>[28x]LMSDWEDEDLDTDNDNIPDSYERNGYTIKDLIAVKWEDSFAEQGYKKYVSNYLESNTAGDPYTDYEKASGSFDKAIKTEARDPLVAAYPIVGVGMEKLIISTNEHASTDQGKTVSRATTNSKTESNTAGVSVNVGYQNGFTANVTTNYSHTTDNSTAVQDSNGESWNTGLSINKGESAYINANVRYYNTGTAPMYKVTPTTNLVLDGDTLSTIKAQENQIGNNLSPGDTYPKKGLSPLALNTMDQFSSRLIPINYDQLKKLDAGKQIKLETTQVSGNFGTKNSSGQIVTEGNSWSDYISQIDSISASIILDTENESYERRVTAKNLQDPEDKTPELTIGEAIEKAFGATKK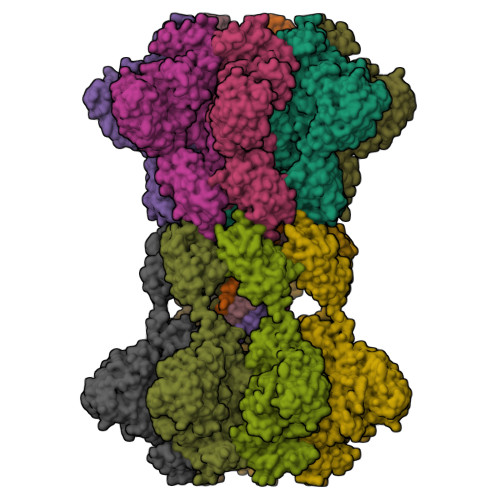DGLLYFNDIPIDESCVELIFDDNTANKIKDSLKTLSDKKIYNVKLERGMNILIKTPTYFTNFDDYNNYPSTWSNVNTTNQDGLQGSANKLNGETKIKIPMSELKPYKRYVFSGYSKDPLTSNSIIVKIKAKEEKTDYLVPEQGYTKFSYEFETTEKDSSNIEITLIGSGTTYLDNLSITELNSTPEILDEPEVKIPTDQEIMDAHKIYFADLNFNPSTGNTYINGMYFAPTQTNKEALDYIQKYRVEATLQYSGFKDIGTKDKEMRNYLGDPNQPKTNYVNLRSYFTGGENIMTYKKLRIYAITPDDRELLVLSVD(5S)-N-[(3S)-7-methoxy-1-methyl-2-oxo-2,3,4,5-tetrahydro-1H-pyrido[3,4-b]azepin-3-yl]-5-phenyl-6,7-dihydro-5H-pyrrolo[1,2-b][1,2,4]triazole-2-carboxamide 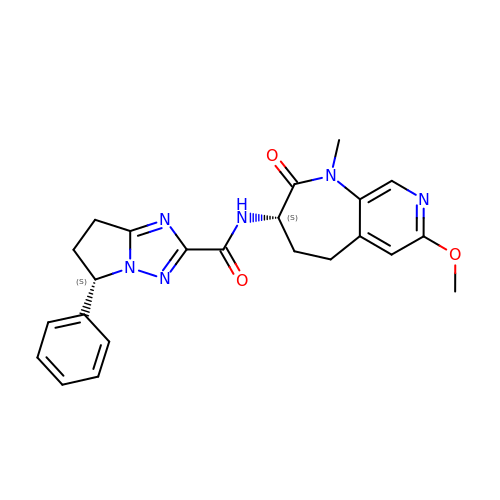| C23 H24 N6 O3 | JXFYROJRZJPKTQ-IRXDYDNUSA-N>[4x]GPTAAALERLTTEEVQGLSDVKTLVNQLYEALNVREHQLQKEVELTTQLETLQQELLPLEEKKLELEQVANRRSNWMAWAGLGLMSVQFGILARLTWWEYSWDIMEPVTYFVTYGTAMAAYAYFVLTREEYILNDVRDRQQLLLLHKKAKKTGFDVNQYNVLKDQIAKLELDLKRLRDPLKLRLPPKAAAKEEGGWSHPQFEK;>[3x]GPTAAALETAVYSKSGGLLPEPHRTSFGIIRLILTVVPGLLIGAAISKNIANFLEENDLFVPSDDDDDDD;> GPTAAALEPHPEEKKKKRSGFRDRKVMEYENRIRAYSTPDKIFRYFATLKVISEPGEAEVFMTPEDFVRSITPNEKQPEHLGLDQYIIKRFDGKKISQEREKFADEGSIFYTLGECGLISFSDYIFLTTVLSTPQRNFEIAFKMFDLNGDGEVDMEEFEQVQSIIRSQTSMGMRHRDRPTTGNTLKSGLCSALTTYFFGADLKGKLTIKNFLEFQRKLQHDVLKLEFERHDPVDGRITERQFGGMLLAYSGVQSKKLTAMQRQLKKHFKEGKGLTFQEVENFFTFLKNINDVDTALSFYHMAGASLDKVTMQQVARTVAKVELSDHVCDVVFALFDCDGNGELSNKEFVSIMKQRLMRGLEKPKDMGFTRLMQAMWKCAQETAWDFALPKQSNW;> HHSRVSVAARDGSFTVSAQKNVEHGIIYIGKPSLRKQRFMQFSSLEHEGEYYMTPRDFLFSVMFEQMERKTSVKKLTKKDIEDTLSGIQTAGCGSTFFRDLGDKGLISYTEYLFLLTILTKPHSGFHVAFKMLDTDGNEMIEKREFFKLQKIISKQDDLMTVKTNETGYQEAIVKEPEINTTLQMRFFGKRGQRKLHYKEFRRFMENLQTEIQEMEFLQFSKGLSFMRKEDFAEWLLFFTNTENKDIYWKNVREKLSAGESISLDEFKSFCHFTTHLEDFAIAMQMFSLAHRPVRLAEFKRAVKVATGQELSNNILDTVFKIFDLDGDECLSHEEFLGVLKNRMHRGLWVPQHQSIQEYWKCVKKESIKGVKEVWKQAGKGLF

The mitochondrial calcium uniporter is a highly selective multi-subunit Ca2+ channel of the inner mitochondrial membrane that serves as the major conduit for uptake of Ca2+ by mitochondria and controls ATP production in response to cytosolic Ca2+ signals. The protein MCU constitutes the pore of the uniporter through which Ca2+ ions flow and EMRE, a small transmembrane protein that associates with MCU, is necessary for Ca2+ uptake in metazoan organisms. Ca2+-dependent control is conferred by proteins that are unique to the uniporter − heterodimers of MICU1-MICU2 in most cells and of MICU1-MICU3 in neurons. At the ~100 nM resting level of [Ca2+]cytosol, MICU1-MICU2 and MICU1-MICU3 heterodimers prevent ion conduction through the channel, and they permit it when Ca2+ levels rise.

Here, we present a 3.3 Å resolution cryo-EM structure of the MCU-EMRE-MICU1-MICU2 assembly, hereafter referred to as the holocomplex, under resting [Ca2+] conditions. Cryo-EM data were collected using a low (<1 nM) concentration of Ca2+ in order to investigate the resting state of the holocomplex. Images containing one MICU1-MICU2 heterodimer per channel yielded a 3D reconstruction of the holocomplex at 3.3 Å resolution. MICU1 and MICU2 associate as a heterodimer and bind to the surface of the channel at the IMS entrance of its pore. Interactions with the channel are mediated solely by MICU1; MICU2 makes no visible contacts with MCU or EMRE. The conformation of the pore is indistinguishable from that observed in a cryo-EM structure of TcMCU-EMRE without MICU1-MICU2 (Wang et al., 2020), which suggests that unlike gating conformational changes in many other ion channels, control by MICU1-MICU2 is not accomplished through motions of pore-lining helices. Strong density that we assign as Ca2+ on the basis of its coordination and analogy to other structures of MCU is present within the ‘E’ ring. Three EMRE subunits are observed at the periphery of the TMD (EMRE 1–3). The mouth of the pore is coordinated by Lys 126 and Arg 129 from α2, and Ser 122 of the α1-α2 turn through a network of hydrogen bonds that involves three of the four MCU-Asp 261 residues of the ‘D’ ring. The structure of the holocomplex and its similarity to a pore-blocking toxin complex indicate that MICU1 binding inhibits the flow of Ca2+ ions by both obstructing the IMS entrance of the pore and by shielding the negative charge of the ‘D’ ring through coordination with basic amino acids.>GGHMTRRGKIVCTLGPATQRDDLVRALVEAGMDVARMNFSHGDYDDHKVAYERVRVASDATGRAVGVLADLQGPKIRLGRFASGATHWAEGETVRITVGACEGSHDRVSTTYKRLAQDAVAGDRVLVDDGKVALVVDAVEGDDVVCTVVEGGPVSDNKGISLPGMNVTAPALSEKDIEDLTFALNLGVDMVALSFVRSPADVELVHEVMDRIGRRVPVIAKLEKPEAIDNLEAIVLAFDAVMVARGDLGVELPLEEVPLVQKRAIQMARENAKPVIVATQMLDSMIENSRPTRAEASDVANAVLDGA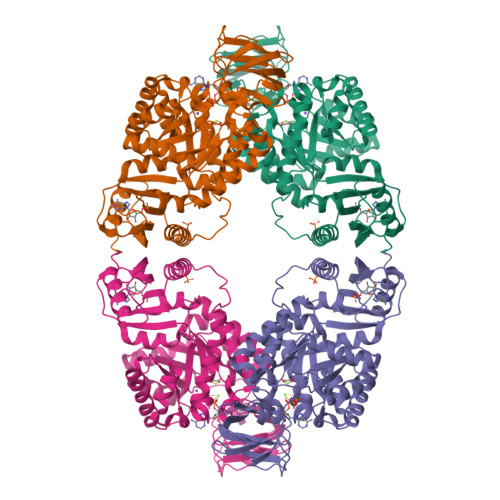DALMLSGETSVGKYPLAAVRTMSRIICAVEENSTAAPPLTHIPRTKRGVISYAARDIGERLDAKALVAFTQSGDTVRRLARLHTPLPLLAFTAWPEVRSQLAMTWGTETFIVPKMQSTDGMIRQVDKSLLELARYKRGDLVVIVAGAPPGTVGSTNLIHVHRIGEDDV[4x]> AEIYNKDGNKVDLYGKAVGLHYFSKGNGENSYGGNGDMTYARLGFKGETQINSDLTGYGQWEYNFQGNNSEGADAQTGNKTCLAFAGLKYADVGSFDYGRNYGVVYDALGYTDMLPEFGGDTAYSDDFFVGRVGGVATYRNSNFFGLVDGLNFAVQYLGKNERDTARRSNGDGVGGSI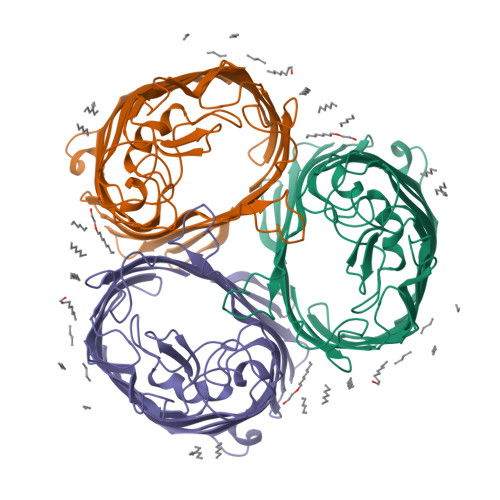SYEYEGFGIVGAYGAADRTNLQEAQPLGNGKKAEQWATGLKYDANNIYLAANYGETRNATPITNKFTNTSGFANKTQDVLLVAQYQFDFGLRPSIAYTKSKAKDVEGIGDVDLVNYFEVGATYYFNKNMSTYVDYIINQIDSDNKLGVGSDDTVAVGIVYQF> MSWQSYVDDHLMCDVEGNH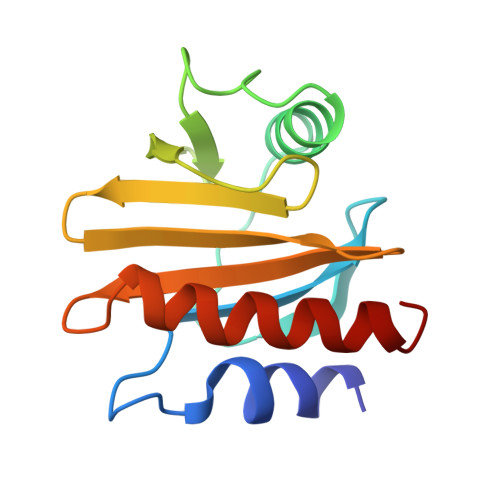LTAAAILGQDGSVWAQSAKFPQLKPQEIDGIKKDFEEPGFLAPTGLFLGGEKYMVIQGEQGAVIRGKKGPGGVTIKKTNQALVFGFYDEPMTGGQCNLVVERLGDYLIESEL> MSYIPG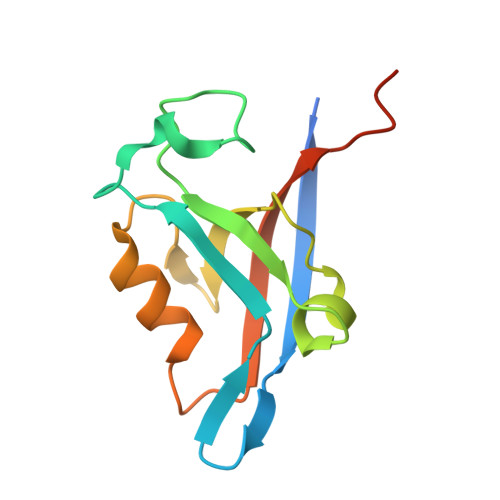QPVTAVVQRVEIHKLRQGENLILGFSIGGGIDQDPSQNPFSEDKTDKGIYVTRVSEGGPAEIAGLQIGDKIMQVNGWDMTMVTHDQARKRLTKRSEEVVRLLVTRQSLQKAVQQSMLS> IPPPPPLPGVAS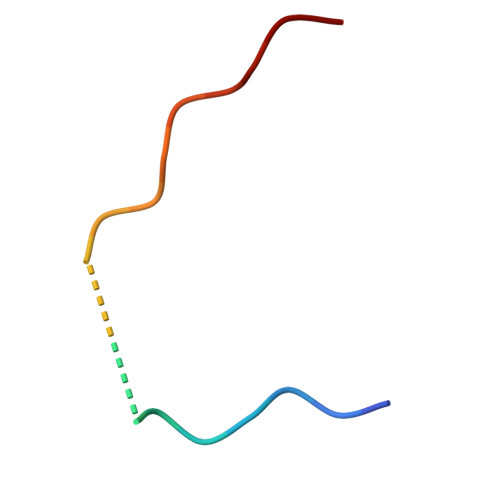IPPPPPLPG> SEMASEIHMTGPMCLIENTNGRLMANPEALKILSAITQPMVVVAIVGLYRTGKSYLMNKLAGKKKGFSLGSTVQSHTKGIWMWCVPHPKKPGHILVLLDTEGLGDVEKGDNQNDSWIFALAVLLSSTFVYNSIGTINQQAMDQLYYVTELTHRIRSKSSPDENENEVEDSADFVSFFPDFVWTLRDFSLDLEADGQPLTPDEYLTYSLKLKKGTSQKDETFNLPRLCIRKFFPKKKCFVFDRPVHRRKLAQLEKLQDEELDPEFVQQVADFCSYIFSNSKTKTLSGGIQVNGPRLESLVLTYVNAISSGDLPCMENAVLALAQIENSAAVQKAIAHYEQQMGQKVQLPTETLQELLDLHRDSEREAIEVFIRSSFKDVDHLFQKELAAQLEKKRDDFCKQNQEASSDRCSALLQVIFSPLEEEVKAGIYSKPGGYRLFVQKLQDLKKKYYEEPRKGIQAEEILQTYLKSKESMTDAILQTD;> SGRPMTYADYFSAWDKWEKQALPGEERDEAVSRLKECLINNSDELRLDRLNLSSLPDNLPAQITLLNVSYNQLTNLPELPVTLKKLYSASNKLSELPVLPPALESLQVQHNELENLPALPDSLLTMNISYNEIVSLPSLPQALKNLRATRNFLTELPAFSEGNNPVVREYFFDRNQISHIPESILNLRNECSIHISDNPLSSHALPALQRLTSSPDYHGPRIYFSMSDGQQNTLHR

The guanylate-binding proteins (GBPs) play critical roles in cell-autonomous immunity against a diverse range of bacterial, viral, and protozoan pathogens. GBP1 contains an N-terminal large GTPase (LG) domain and a C-terminal helical region, which can be further divided into a middle domain (MD) that contains the α7-α11 helices and a GTPase effector domain (GED) that consists of the α12-α13 helices. The GED folds back and interacts with LG and MD, which is important to maintain GBP1 at the resting state. Recent studies have discovered that IpaH9.8 ubiquitinates and degrades a subset of GBPs, which is important for S. flexneri to suppress host defense and replicate in the cells.

We subsequently crystallized the LG-MD region of GBP1 (GBP1LG-MD) in complex with IpaH9.8LRR and determined the structure at 3.6 Å. In the complex structure, it engages GBP1LG using the concave surface of the solenoid. Three regions in GBP1LG are involved in interacting with IpaH9.8LRR: the P-loop, the switch II region, and the α3 helix. On the other hand, these regions are involved in forming the dimer interface in the LG dimer structure, and therefore binding of IpaH9.8 would lead to the disruption of the GBP1LG dimer. In the structure, seven out of the eight LRR modules in IpaH9.8LRR contribute residues to interact with GBP1. The residues involved in binding GBP1 are unique to IpaH9.8, explaining the fact that only IpaH9.8, but not other IpaH proteins, specifically degrades the GBPs. In our structure, since the GED domain is not present, the MD domain is free to adopt a relaxed conformation. The α7 helix, which is forced to bend in the apo structure due to the interaction between the GED and the LG-MD domains, springs back to the straightened state. Starting from a highly conserved Gln321, the C-terminal half of the α7 helix rotates ~13°, and this conformational change is transmitted toward the rest of the protein, causing an ~20° en bloc rotation of the α8-α11 helices. In contrast, the GBP1LG-MD structure likely reflects GBP1 at its most relaxed state.>MEAGITGTWYNQLGSTFIVTAGADGALTGTYVTARGNAESRYVLTGRYDSAPATDGSGTALGWTVAWKNNYRNAHSATTW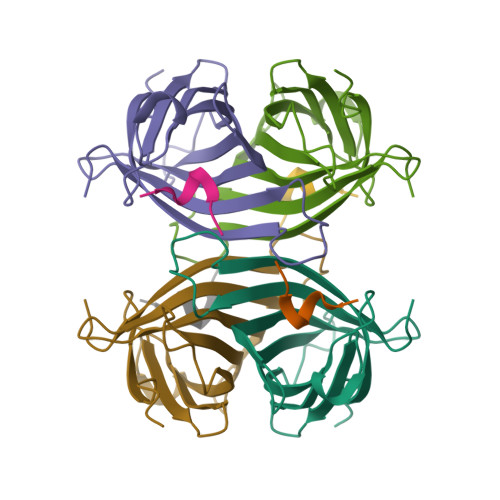SGQYVGGAEARINTQWLLTSGTTEYNAFMSTLVGHDTFTKVKPSAAS[2x];>[2x]SAWSHPQFEK>[2x]GREEIFQVALHKRDSGEQLGIKLVRRTDEPGVFILDLLEGGLAAQDGRLSSNDRVLAINGHDLKYGTPELAAQIIQASGERVNLTIARPGKPQP;>NLNSSRVPDLLV[2x]

The C-terminus of the severe acute respiratory syndrome coronavirus 2 (SARS-CoV-2) protein E contains a PBM (PDZ-binding motif) targeting PDZ (PSD-95/Dlg/ZO-1) domains, which is identical to the PBM of SARS-CoV. Targeting multiple cellular PDZ (PSD-95/Dlg/ZO-1)-containing proteins through short linear PDZ-binding motifs (PBMs) is a common strategy used by viruses to facilitate their viral replication and dissemination to new hosts. PBMs are mainly located at the C-terminus of target proteins and interact directly with PDZ domains. We solved three crystal structures of complexes between human LNX2, MLLT4, and MPP5 PDZs and SARS-CoV-2 E PBM highlighting its binding preferences for several cellular targets.

LNX2 acts as a molecular scaffold for Numb family proteins, essential players in the regulation of cell adhesion and polarity. The crystal structure of LNX2-PDZ2 in complex with SARS-CoV-2-E-PBM was solved at a resolution of 3.3 Å. Each of the two LNX2-PDZs present in the asymmetric unit are bound to the peptide. Electron density was observed for the last five residues of the two peptides. In both cases, the last three residues of the SARS-CoV-2-E-PBM peptide bind to the canonical α2 helix/β2 strand groove in each PDZ unit. As for MLLT4 and MPP5, the PBM of protein E conventionally binds to the PDZ of LNX2. The C-terminal carboxylate of Val 0 of the PBM forms three hydrogen bonds: two with the amide protons of Leu 351 and Gly 352 of the “GLGF” loop of LNX2-PDZ2 and one with the Ile 353 amide proton. The proton amide of Val 0 also forms an H-bond with the carbonyl of Ile 353. In addition, the amide and carbonyl groups of Leu -2 form hydrogen bonds with the carbonyl and amide proton of Leu 355, respectively. In one of the two complexes, an ionic bond is formed between the carboxylate of Val at position -3 of the PBM and the amine group of Arg 357 at the end of the β2 strand.>HHHHHHMSAIENFDAHTPMMQQYLRLKAQHPEILLFYRMGDFYELFYDDAKRASQLLDISLTKRGASAGEPIPMAGIPYHAVENYLAKLVNQGESVAICEQIGDPATSKGPVERKVVRIVTPGTISDEALLQERQDNLLAAIWQDSKGFGYATLDISSGRFRLSEPADRETMAAELQRTNPAELLYAEDFAEMSLIEGRRGLRRRPLWEFEIDTARQQLNLQFGTRDLVGFGVENAPRGLCAAGCLLQYAKDTQRTTLPHIRSITMEREQDSIIMDAATRRNLEITQNLAGGAENTLASVLDCTVTPMGSRMLKRWLHMPVRDTRVLLERQQTIGALQDFTAGLQPVLRQVGDLERILARLALRTARPRDLARMRHAFQQLPELRAQLETVDSAPVQALREKMGEFAELRDLLERAIIDTPPVLVRDGGVIASGYNEELDEWRALADGATDYLERLEVRERERTGLDTLKVGFNAVHGYYIQISRGQSHLAPINYMRRQTLKNAERYIIPELKEYEDKVLTSKGKALALEKQLYEELFDLLLPHLEALQQSASALAELDVLVNLAERAYTLNYTCPTFIDKPGIRITEGRHPVVEQVLNEPFIANPLNLSPQRRMLIITGPNMGGKSTYMRQTALIALMAYIGSYVPAQKVEIGPIDRIFTRVGAADDLASGRSTFMVEMTE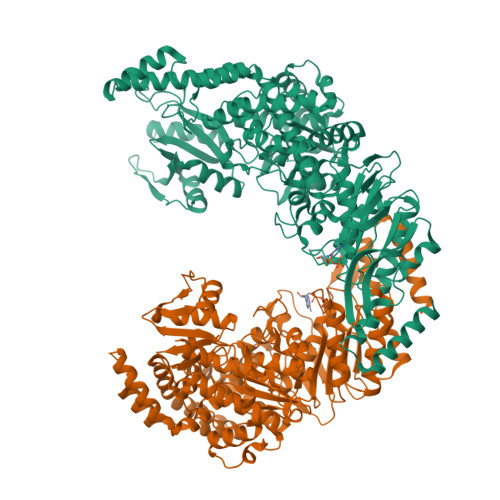TANILHNATEYSLVLMDEIGRGTSTYDGLSLAWACAENLANKIKALTLFATHYFELTQLPEKMEGVANVHLDALEHGDTIAFMHSVQDGAASKSYGLAVAALAGVPKEVIKRARQKLRELESISPNAAATQVDGTQMSLLSVPEETSPAVEALENLDPDSLTPEQALEWIYRLKSLV[2x]>[3x]MKFKHQGLVADLLPNIRVMQGVGHFMFNYYSEGKKFPHRIYCIVTLLLLLLQYGMMAVNLMMESDDVDDLTANTITMLFFLHPIVKMIYFPVRSKIFYKTLAIWNNPNSHPLFAESNARFHALAITKMRRLLFCVAGATIFSVISWTGITFIEDSVKRITDPETNETTIIPIPRLMIRTFYPFNAMSGAGHVFALIYQFYYLVISMAVSNSLDVLFCSWLLFACEQLQHLKAIMKPLMELSATLDTVVPNSGELFKAGSADHLRESQGVQPSGNGDNVLDVDLRGIYSNRQDFTATFRPTAGTTFNGGVGPNGLTKKQEMLVRSAIKYWVERHKHVVRLVTAVGDAYGVALLLHMLTTTITLTLLAYQATKVNGVNVYAATVIGYLLYTLGQVFLFCIFGNRLIEESSSVMEAAYSCHWYDGSEEAKTFVQIVCQQCQKAMSISGAKFFTVSLDLFASVLGAVVTYFMVLVQLK;> MARLVLHEVRYVLMAMLYISRGMAKQIQNSTIDLYVYWFLTFIPIASLCVPQFTYLVVDTKSLIDFISVLVPITEILLTNGKMIICNVKRGKIINLINQVQVAWDECAKSEHLEIQTLITATAKKTKIFVIIYTTSFLLICVEYSSMPLFKLIYHSAVYGKQSNYTIALPYLSRFAYSTESTTSFAWTYFFILLGVYLLALTLSGFDSLFATLVMHVKMMFKVLKFEIEQLGLDLSAGKSHVELQAKLKQIILKHKTNLSLIEQLEDGFSFFLMAQFLTSSILVCVVLYELTMVFGWNEDTFKTVTYLPGAILQLFLFCWYAQQITEEARLVSDHIYNIPWYLADPKLQKDILTFMVKAQKPTGVTASKFYMVTLQTFQRISSTSYSYFTLLQTINQQ

Most insects, including human-targeting mosquitoes, detect odors through odorant-activated ion channel complexes consisting of a divergent odorant-binding subunit (OR) and a conserved co-receptor subunit (Orco). As a basis for understanding how odorants activate these heteromeric receptors, we report here cryo-EM structures of two different heteromeric odorant receptor complexes containing ORs from disease-vector mosquitos Aedes aegypti or Anopheles gambiae. We determined the structure of a heteromeric complex formed by ORs from these species in complex with a Apocrypta bakeri fig wasp Orco that is amenable to structural determination. We find that these complexes form asymmetric tetramers containing 1 OR and 3 Orco subunits, where activation of the sole OR subunit upon ligand binding suffices to open the ion conduction pathway.

To determine if the 1:3 subunit stoichiometry can be observed with other members of the OR family, we turned to studying the OR28 receptor of An. gambiae, a main vector of malaria, that responds to the natural odorants acetophenone (a plant volatile) and 2,4,5-trimethylthiazole (henceforth TMT; an animal odor, originally isolated from anal secretions of mammals). A different heteromeric OR/Orco complex also has a 1:3 subunit stoichiometry and a similar mode of channel activation. Overall, subunit stoichiometry, mechanism of pore opening and ligand binding of the AgOR28/Orco complex largely resembles the observations of the AaOR10/Orco complex, suggesting that these might be conserved features of this family of proteins.> MPTQKELRDTMSKKLQEAIKHPDPAVVAGRKSAIKRWVGVLQDNFMEHIKYFKGDKLKFLHNVFQDEGCWSGVRLDNAALGQRFTEEKIGGIDNPLRKYEMACSYCVVDKIHPLFQKRFESYRNKFPPGAFDGKTETEFGKYVRNSLLDSIKRKGPVFDFWIDRESGELKKYDAVEGFDSAVKFKWSEGVEYFYNHLKEEDKEKKLTEAILALSRVQSVEKDAPILDFCVNKIVDKDTLLQKLSQKDKGVYSLFVELIESCFFDTVHDLVQCWCYKEVSAGGDHSEKIFSQRDYELFLSSLSDTMLKNPELSVQARSLIMEFWECGSLYQYRKAAVNTSNYTVPTSGVFAELIVNWRREDIYKTDEEKEIEKKEILDMMSFAKDCFPEKFELFKKLIIRDLRLCGREGKRVNVDYGLFAEELFSELEKTILPPGPVGDGPCSNLRSRSKAHGSKKTTLPVDDSPQSELGTPSVSGVSSYKKKSVFTLSGNKLEHHHHHH;> MSNGDGLIRSLVDGDLEGFRQGFESFLDQCPSFLYHVSAGRFLPVFFFSMFSTAHDANILNANERVYFRFDNHGVNPRNGENRNTANLKVAVYRDGQQVVRCYSISDRPNSDGLRFSTRERNALVQEIRRQNPNLREEDLNFEQYKVCMHGKGKSQGEAIATVFEVIREKDRQGRDKFAKYSASEINLIRRLLGDHRLTIKEIEGRQLNQNQLRQLGRLVNFAQVAQGQQGIDNFMEMLASDRRQDVRDRIRREILPYITDIYNNYRQVLENNIENRNQRFEGHGFLLGFLANFSHRYTIGVDLDLSPRNSHVAFLVRHQVERENIPIVINLATRAPPYIALNRARSHAERLHVFSFIPIHTESRNTVCVGLNFNLNLDPFSVDTVGLQQDRFPLVQRLFECLENEGIRENIRDFLLHHLPAEIPRNAENYDRIFDCITGFAFGNSAFDRHPLELEEEDEAPITKYIFRHGDEGLRCLTMVFHAEGSDIVILHIRAHDAQQQGAINLQTLNVNGNDVHVWEVSCTLNNQLELDIDLPNDLGLYHDYQNNNANNFLAGDLVQVPNTENVHNTLNQVVNDGWKNIAQHRGLFQEISGALMPLVDTINVNSEDKFRSILHGTFYASDNPYKVLAMYKVGQTYSLKRGQEEEGERVILTRITEQRLDLLLLRQPRENDLDTHPIGYVLRLANNAEEVGQQQNDARQEIGRLKKQHRGFIPITSGNEVVLFPIVFNRDAHEAGNLILFPEGIGREEHVHRLDRHVRLEHHHHHH

Cytoplasmic incompatibility (CI) results when Wolbachia bacteria-infected male insects mate with uninfected females, leading to embryonic lethality. CI is caused by linked pairs of Wolbachia genes called CI factors (CifA and CifB). Protein-binding experiments and expression of cif genes in yeast have shown that CifA binds its cognate CifB specifically and rescues CifB-induced yeast growth defects. CidBwMel consists of a region, which is predicted to contain two PD-(D/E)XK (pseudo) nuclease domains (residue 1-751; hereafter CidBwMelND1-ND2, ND: nuclease domain) and a C-terminal deubiquitylase (DUB) domain.

Of note, the ND1-ND2 region of CidBwPip_I(b/2) (a CidBwMel ortholog from the Wolbachia strain wPip Tunis line, hereafter CidBwPip(Tunis)ND1-ND2) expressed well in E. coli and shares a sequence identity of 71% with CidBwMelND1-ND2. We successfully determined a crystal structure of CidBwPip(Tunis)ND1-ND2 in complex with CidAwPip(Tunis) (specifically CidAwPip_I(γ/2)32). The structure of CidBwPip(Tunis)ND1-ND2 is very similar to the model for CidBwMelND1-ND2. (The residues at the interface are well resolved in CidAwPip(Tunis)-CidBwPip(Tunis)ND1-ND2 with good electron density). Substituting the CidAwPip(Tunis) residues at its CidB-binding interface with the corresponding ones from CidAwMel abolished its ability to bind CidBwPip(Tunis)ND1-ND2 and neutralize the CidBwPip(Tunis)-induced growth defect in yeast. Thus, the structure of the CidAwPip(Tunis)-CidBwPip(Tunis)ND1-ND2 complex accurately captures the CidA-CidB interaction mode and is biologically relevant. Among the positions that show divergence, residues 118, 125, 149, 150, 341, 342, 399, and 400 of CidAwPip and residues 242, 243, 253, 254, 257, 451, 452, 460, 461, and 462 of CidBwPip map to the binding interface of the two proteins. These variations create distinct interaction surfaces for each of the four known CidAwPip_I variants. Similarly, each of the four CidBwPip_I variants has a unique combination of residues at the CidA-binding interface. His-tagged CidA variants I(α/1), I(γ/1), I(β/2), and I(γ/2) cannot pull down GST-tagged CidB variants I(b/2), I(b/1), I(a/2), and I(a/1), respectively, which supports the hypothesis that natural sequence variations affect binding interactions between CidAwPip and CidBwPip from different strains.> EEWLDILGNGLLRKKTLVPGPPGS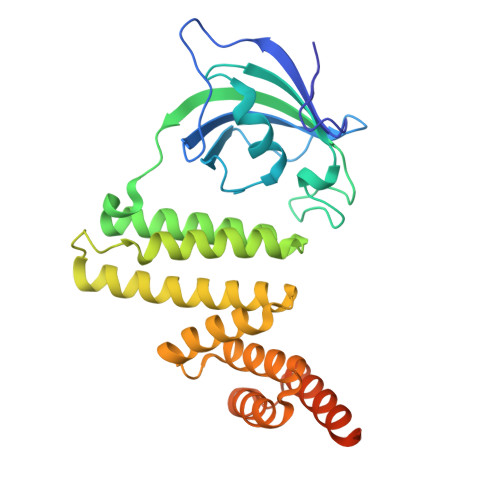SRPVKGQVVTVHLQTSLENGTRVQEEPELVFTLGDCDVIQALDLSVPLMDVGETAMVTADSKYCYGPQGRSPYIPPHAALCLEVTLKTAVDGPDLEMLTGQERVALANRKRECGNAHYQRADFVLAANSYDLAIKAITSSAKVDMTFEEEAQLLQLKVKCLNNLAASQLKLDHYRAALRSCSLVLEHQPDNIKALFRKGKVLAQQGEYSEAIPILRAALKLEPSNKTIHAELSKLVKKHAAQRSTETALYRKMLGNPSRLPAKCPG>[2x]MNAGHQLRLGVAGLGRAFTLMLPTLQQDPRIKLVAACDPRGSARAQFASDFRAPVYPDIEGLASNPDVEAIYIASPHQFHAQQARIAARHGKHVLVEKPMALSLGDCDEMIQHCRD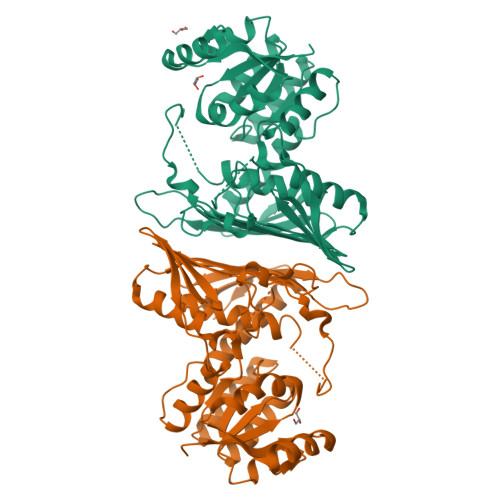AGVHLIVGHCHSFDTPYLSAREIVQSGELGPVRMVHALNYTDFLYRPRRPEELRTEEGGGVVFSQAAHQVDIVRLLVGTRVRRVRAITGDWDPMRPTQGAYSALLWFEGGAFASISYNGYGHFDSDEWCDWIGEMGGDKSPEAYGAARRKLATVGSAQEEANLKAAATYGGPGYVAAATDAQPIWHQHFGPIVVSCERGDIRPLPDSVCVYADLAKERRSLQRPVVPRFEVIDELYHAVVNEIKPLHDGVWARATLEVCLALLDSAGSGKDVELPR>MAFYSCCWVLLALTWHTSAYGPDQRAQKKGDIILGGLFPIHFGVAAKDQDLKSRPESVECIRYNFRGFRWLQAMIFAIEEINSSPALLPNLTLGYRIFDTCNTVSKALEATLSFVAQNKIDSLNLDEFCNCSEHIPSTIAVVGATGSGVSTAVANLLGLFYIPQVSYASSSRLLSNKNQFKSFLRTIPNDEHQATAMADIIEYFRWNWVGTIAADDDYGRPGIEKFREEAEERDICIDFSELISQYSDEEEIQHVVEVIQNSTAKVIVVFSSGPDLEPLIKEIVRRNITGKIWLASEAWASSSLIAMPQYFHVVGGTIGFALKAGQIPGFREFLKKVHPRKSVHNGFAKEFWEETFNCHLQEGAKGPLPVDTFLRGHEESGDRFSNSSTAFRPLCTGDENISSVETPYIDYTHLRISYNVYLAVYSIAHALQDIYTCLPGRGLFTNGSCADIKKVEAWQVLKHLRHLNFTNNMGEQVTFDECGDLVGNYSIINWHLSPEDGSIVFKEVGYYNVYAKKGERLFINEEKILWSGFSREVPFSNCSRDCLAGTRKGIIEGEPTCCFECVECPDGEYSDETDASACNKCPDDFWSNENHTSCIAKEIEFLSWTEPFGIALTLFAVLGIFLTAFVLGVFIKFRNTPIVKATNRELSYLLLFSLLCCFSSSLFFIGEPQDWTCRLRQPAFGISFVLCISCILVKTNRVLLVFEAKIPTSFHRK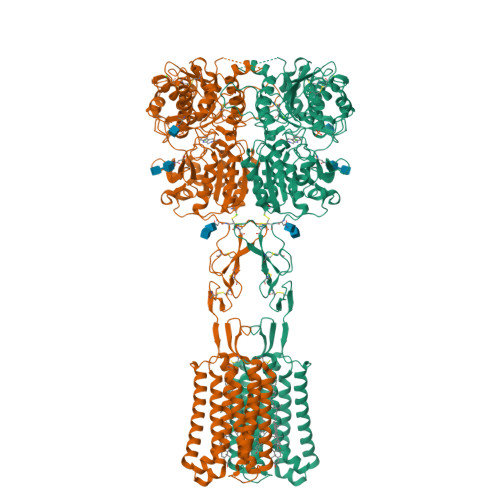WWGLNLQFLLVFLCTFMQIVICVIWLYTAPPSSYRNQELEDEIIFITCHEGSLMALGFLIGYTCLLAAICFFFAFKSRKLPENFNEAKFITFSMLIFFIVWISFIPAYASTYGKFVSAVEVIAILAASFGLLACIFFNKIYIILFKPSRNTIEDYKDDDDK[2x]> MRGSHHHHHHGMASMRILLSNDDGVHAPGIQTLAKALREFADVQVVAPDRNRSGASNSLTLESSLRTFTFDNGDIAVQMGTPTDCVYLGVNALMRPRPDIVVSGINAGPNLGDDVIYSGTVAAAMAGRHLGFPALAVSLNGYQHYDTAAAVTCALLRGLSREPLRTGRILNVNVPDLPLAQVKGIRVTRCGSRHPADKVIPQED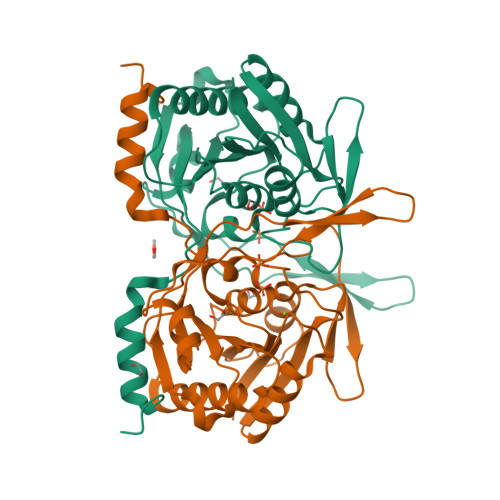PRGNTLYWIGPPGDKYDAGPDTDFAAVDEGYVSVTPLHVDLTAHSAHDVVSDWLDSVGVGTQW>[2x]MAATRDVTHLTDISKG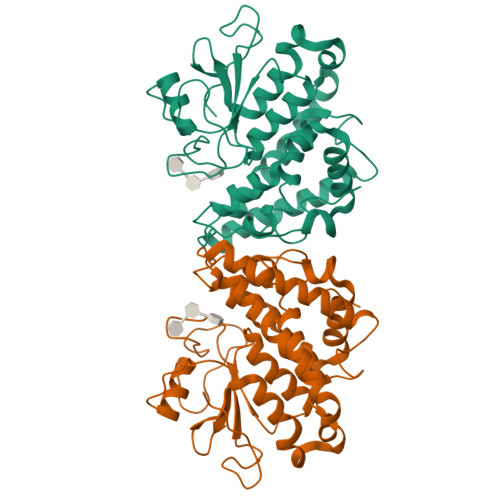LAEADGSFKRKASTFRRFIEKGGEFEPEKGRYHLYVAYSSPWATRTLIVRKIKGLEEIVGVTIVSPLFSAHGWPFGDVSPFPGAEADPFYNAQYVRDLYLRADPKYEGRFTVPVLWDKKTETVVNNESSEIIRIFNTAFNEFLPADKAAIHLYPEALKSEIDEINEWVYDTVNNGVYKAGFATTQQAYEAAVIPLFESLDRLEKILTGKDYLVGDQLTEADVRLFVTIIRFDPAYVGHFKCNLRTIRDGYPAIHLWLRKLYWNNSAFSETCKFDHIKASYYAQKNVNPTLVVPLGPIPNILPLHHHHHH>GSHMGSQFWVTSQKTEASERCGLQGSYILRVEAEKLTLLTLGAQSQILEPLLFWPYTLLRRYGRDKVMFSFEAGRRCPSGPGTFTFQTSQGNDIFQAVEAAIQQQKAQGKVGQAQDILRLEHHHHHH[2x];>[2x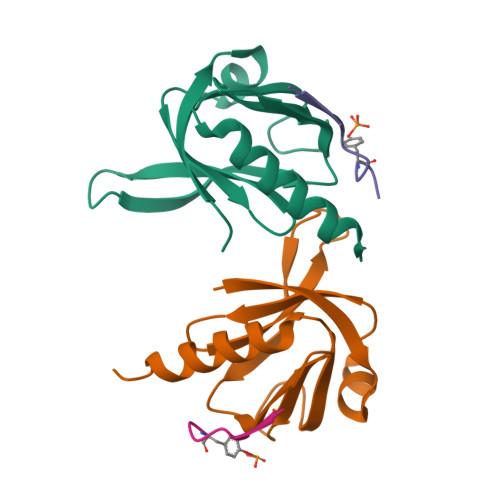]STWIENKLYGMSD>[3x]MSLPHCETLLLEPIEGVL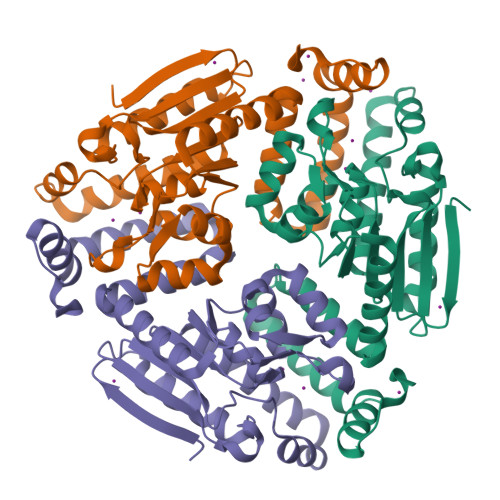RITLNRPQSRNAMSLAMVGELRAVLAAVRDDRSVRALVLRGADGHFCAGGDIKDMAGARAAGAEAYRTLNRAFGSLLEEAQAAPQLLVALVEGAVLGGGFGLACVSDVAIAAADAQFGLPETSLGILPAQIAPFVVRRIGLTQARRLALTAARFDGREALRLGLVHFCEADADALEQRLEETLEQLRRCAPNANAATKALLLASESGELGALLDDAARQFAEAVGGAEGSEGTLAFVQKRKPVWAQGSHHHHHH> SMMSPNPLQKPAI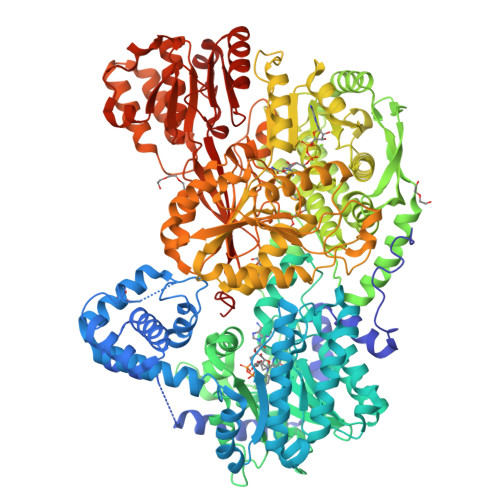DAAPAPFADFAPPVRPQSTLRRAITAAYRRPETECLPPLVEAATQSKEIRDAAASTARKLIEALRGKHSGSGVEGLVQEYSLSSQEGVALMCLAEALLRIPDTATRDALIRDKIADGNWKSHLGGSRSLFVNAATWGLVVTGKLTSTVNDRSLAAALTRLISRCGEPVIRRGVDMAMRMMGEQFVTGETIREALKRSKELEEKGFSYSYDMLGEAATTAADAERYYRDYESAIHAIGKASAGRGIYEGPGISIKLSALHPRYSRAQAARVMGELLPRVKALALLAKNYDIGLNIDAEEADRLELSLDLLEVLCLDGDLSGWNGMGFVVQAYGKRCPFVLDFIIDLARRSGRRIMVRLVKGAYWDAEIKRAQLDGLADFPVFTRKIHTDVSYIACAAKLLAATDVVFPQFATHNAQTLAAIYHMAGKDFHVGKYEFQCLHGMGEPLYEEVVGRGKLDRPCRIYAPVGTHETLLAYLVRRLLENGANSSFVHRINDPKVSIDELIADPVEVVRAMPVVGAKHDRIALPAELFGDARTNSAGLDLSNEETLASLTEALRESAAMKWTALPQLATGPAAGETRTVLNPGDHRDVVGSVTETSEEDARRAVRLAADAAPDWAAVPPSERAACLDRAAELMQARMPTLLGLIIREAGKSALNAIAEVREAIDFLRYYAEQTRRTLGPGHGPLGPIVCISPWNFPLAIFTGQIAAALVAGNPVLAKPAEETPLIAAEGVRILREAGIPASALQLLPGDGRVGAALVAAAETAGVMFTGSTEVARLIQAQLADRLSPAGRPIPLIAETGGQNAMIVDSSALAEQVVGDVITSAFDSAGQRCSALRVLCLQEDVADRILTMLKGALHELHIGRTDRLSVDVGPVITSEAKDNIEKHIERMRGLGRKVEQIGLASETGVGTFVPPTIIELEKLSDLQREVFGPVLHVIRYRRDDLDRLVDDVNATGYGLTFGLHTRLDETIAHVTSRIKAGNLYINRNIIGAVVGVQPFGGRGLSGTGPKAGGPLYLGRLVTTAPVPPQHSSVHTDPVLLDFAKWLDGKGARAEAEAARNAGSSSALGLDLELPGPVGERNLYTLHARGRILLVPATESGLYHQLAAALATGNSVAIDAASGLQASLKNLPQTVGLRVSWSKDWAADGPFAGALVEGDAERIRAVNKAIAALPGPLLLVQAASSGEIARNPDAYCLNWLVEEVSASINTAAAGGNASLMAIG> MAEQLVEAPAYARTLDRAVEYLLSCQKDEGYWWGPLLSNVTMEAEYVLLCHILDRVDRDRMEK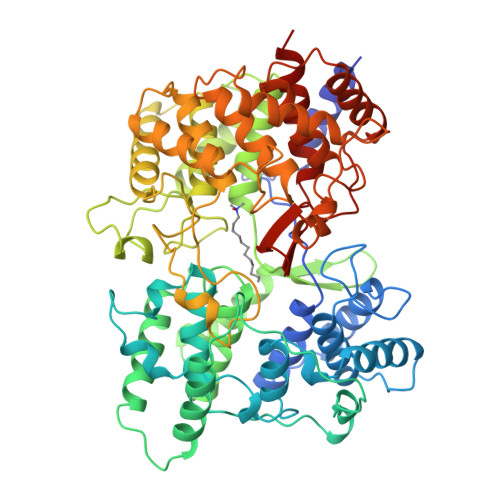IRRYLLHEQREDGTWALYPGGPPDLDTTIEAYVALKYIGMSRDEEPMQKALRFIQSQGGIESSRVFTRMWLALVGEYPWEKVPMVPPEIMFLGKRMPLNIYEFGSWARATVVALSIVMSRQPVFPLPERARVPELYETDVPPRRRGAKGGGGWIFDALDRALHGYQKLSVHPFRRAAEIRALDWLLERQAGDGSWGGIQPPWFYALIALKILDMTQHPAFIKGWEGLELYGVELDYGGWMFQASISPVWDTGLAVLALRAAGLPADHDRLVKAGEWLLDRQITVPGDWAVKRPNLKPGGFAFQFDNVYYPDVDDTAVVVWALNTLRLPDERRRRDAMTKGFRWIVGMQSSNGGWGAYDVDNTSDLPNHIPFCDFGEVTDPPSEDVTAHVLECFGSFGYDDAWKVIRRAVEYLKREQKPDGSWFGRWGVNYLYGTGAVVSALKAVGIDTREPYIQKALDWVEQHQNPDGGWGEDCRSYEDPAYAGKGASTPSQTAWALMALIAGGRAESEAARRGVQYLVETQRPDGGWDEPYYTGTGFPGDFYLGYTMYRHVFPTLALGRYKQAIERR> MTAPHDVPDLTGSGEYLVPDVLQPGLTLVLVGTAPSGISARARAYYANPENKFWRTLHAVGLTPRQLVPQEYATLPQYGLGLTDVAKRHSGVDAALPGEAWRPDELRRKVEHYRPRIVAFTSKRGASETLGVPTGKLPYGPQPQPLDWPAETELWVLPSTSPLGHNHFRLEPWQALGDRV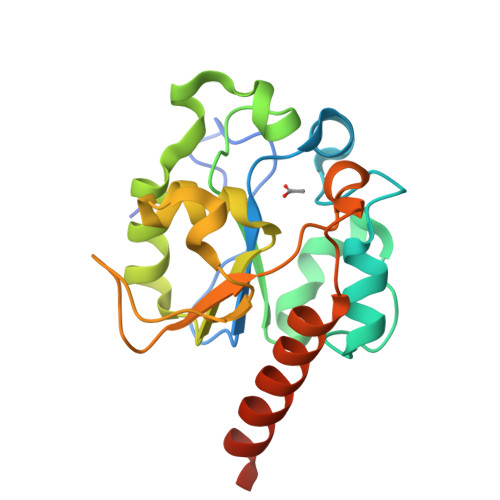RELRGAAEAGNPSPETPVL>[4x]MRIPLVGKDSIESKDIGFTLIHEHLRVFSEAVRQQWPHLYNEDEEFRNAVNEVKRAMQFGVKTIVDPTVMGLGRDIRFMEKVVKATGINLVAGTGIYIYIDLPFYFLNRSIDEI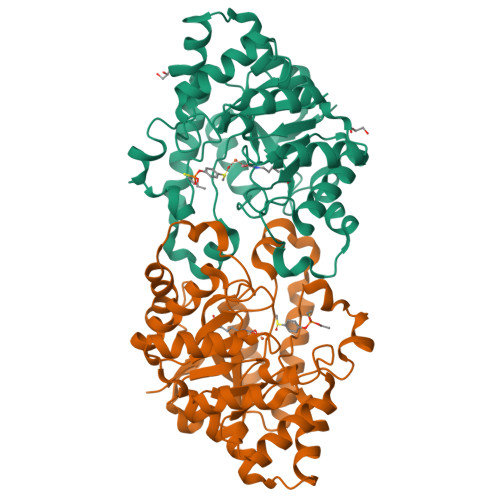ADLFIHDIKEGIQGTLNKAGFVKIAADEPGITKDVEKVIRAAAIANKETKVPIITHSNAHNNTGLEQQRILTEEGVDPGKILIGHLGDTDNIDYIKKIADKGSFIGLDRYGLDLFLPVDKRNETTLRLIKDGYSDKIMISHDYCCTIDWGTAKPEYKPKLAPRWSITLIFEDTIPFLKRNGVNEEVIATIFKENPKKFFS>YNEATIENSTVGGGGYNQAKGRNSTVAGGYNNEATGTDS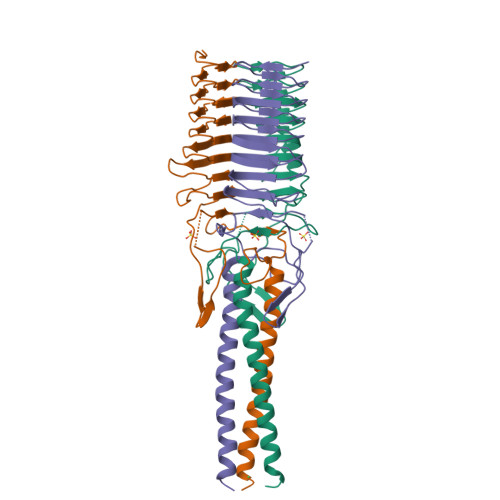TIAGGRKNQATGKGSFAAGIDNKANADNAVALGNKNTIEGENSVAIGSNNTVKKGQQNVFILGSNTDTTNAQNGSVLLGHNTAGKAATIVNSAEVGGLSLTGFAGASKTGNGTVSVGKKGKERQIVHVGAGEISDTSTDAVNGSQLHALATVVAQNKADIKDLDDEVGLLGEEINKHHHHH[3x]>[2x]MRNIRKIKVDNMKVSVYGAGNQNLYINKLNLPEKFGGEPPYGGSRMAIEFAEAGHDVVLAEPNKNIMSDDLWKKVEDAGVKVVSDDVEAAKHGEIHVLFTPFGKATFRIAKTIIEHVPENAVICNTCTVSPVVLYYSLEPILRTKRKDVGISSMHPAAVPGTPQHGHYVIGGKTTDGKELATEEQIKKAVELAKSAGKEAYVVPADVSSVVADMGSLVTAVALSGVLDYY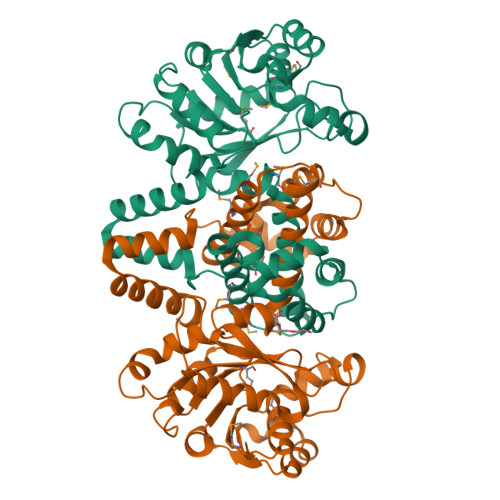TVGRKIINAPKKMIEQQVIMTLQTMASLVETSGIEGMVKALNPELLIRSASSMKLLDRQKDLDAALEILQNLDETLKAEVEKAEIKPTTLVAAQSLVKEIKTLIGGAAAEGAIKRSARKLFEHADPNSSSVDKLAAALEHHHHHH6-amino-1,3,5-triazin-2(1H)-one 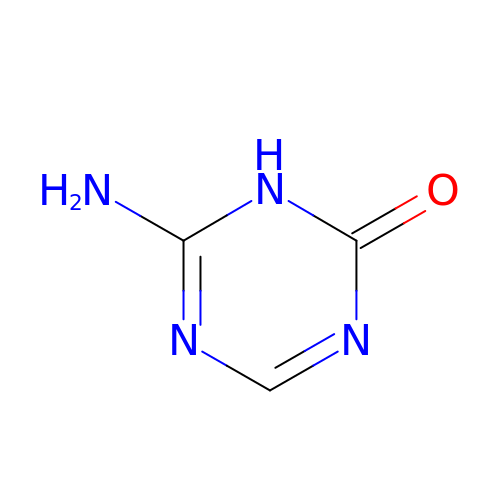| C3 H4 N4 O | MFEFTTYGMZOIKO-UHFFFAOYSA-N> HSDPARRGQLSVCDSISEWVTAADKK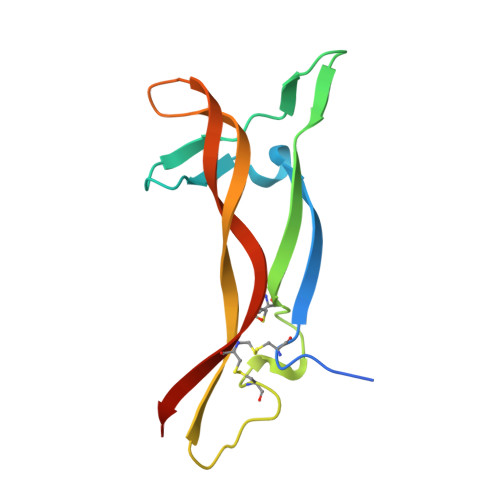TAVDMSGGTVTVLEKVPVSKGQLKQYFYETKCNPMGYTKEGCRGIDKRHWNSQCRTTQSYVRALTMDSKKRIGWRFIRIDTSCVCTLTIKRGR We describe here the use of an artificial cofactor employing the well‐known biotin‐streptavidin system to catalyze a Baylis‐Hillman reaction. As protein host, we chose streptavidin, as it can be easily crystallized and thereby supports the design process. There are several examples using streptavidin as the host for these cofactors, since its natural ligand biotin binds strongly (K d∼10−15 M) and is easy to modify with catalysts at the carboxylic acid group. No enzyme is known to naturally catalyze the Baylis‐Hillman reaction, a very versatile and atom‐economic C−C bond forming reaction for the production of various functionalized compounds and intermediates of active pharmaceutical ingredients (APIs).

We chose a derivative of DMAP as the artificial cofactor due to its low steric demand, which will facilitate its inclusion into the protein scaffold. The protein host around the cofactor was rationally designed on the basis of high‐resolution crystal structures obtained after each variation of the amino acid sequence. The location of the catalyst is in a shallow cavity at the surface of the protein. The system was evolved through repeated cycles of mutagenesis, activity tests, and structure determination. According to the presented structures and calculations the catalytically active site is too shallow to undergo interactions with 1.

> MASMTGGQQMGRDEAGITGTWYNQLGSTFIVTAGADGALTGTYESAAGKAESRYVLTGRYDSAPATDGSGTALGWTVAWKNNYRNAHSATTWSGQYVGGAEARINTQWLLTAGATEANGWASTLVGHDTFTKVKPSAASIDAAKKAGVNNGNPLDAVQQ>[3x]SNAMIDKSAVIHPSSIIEEGAVIGANVRIGPFCVIGSHVEIGEGTDIKSHVVINGHTRIGRDNQIYQFASIGEVNQDLKYRGEPTQVIIGDRNLIRESVTIHRGTTQGGNITKIGNDNLLMINTHVAHDCIIGDRCIIANNGTLGGHVT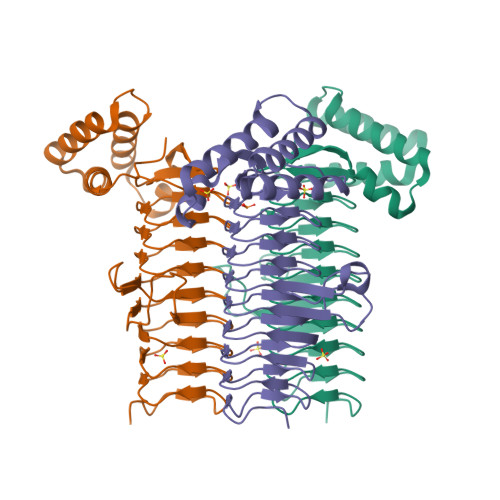LGDYVIIGGMSAVHQFCQIGSHVMVGGCSGVAQDVPPFVIAQGNHATPYGLNIEGLKRRGFAKEDLHAIRNAYKILYRNGKTLEEAREEIAQLAADNNNQYVKIFSDFLENSAKSNRGIIR6-deoxy-1-O-phosphono-beta-L-galactopyranose | C6 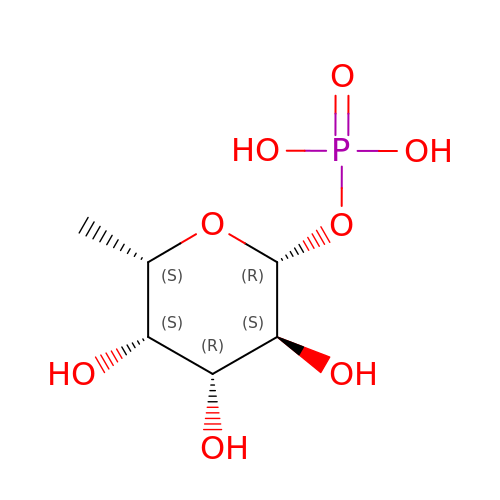H13 O8 P | PTVXQARCLQPGIR-SXUWKVJYSA-N> MNQSDSSLMDLPLEIHLSLLEYVPNELRAVNKYFYVLHNHSYKEKSLAWI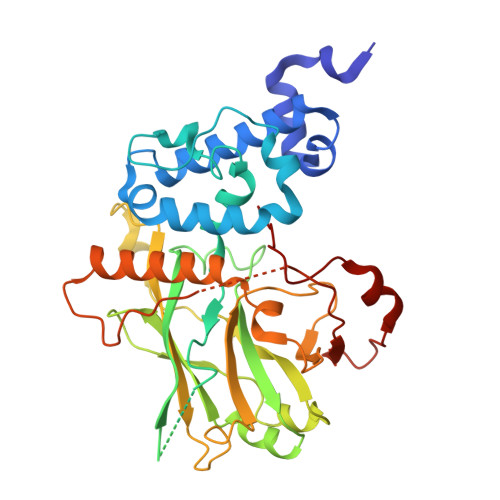AEDNYIWAVVKHSLCLYVKSLDPLRQHAREIIQETKEPGFNVPLCMTKYIADSWYIVYNALQYPGKIINMGWDKYTKSQDLNGSDSTSNFNSRPKERTLMQSLTALPVNFWSRKKDEPTPVNVWFYVKNAHVARYIPKIITEIGICNYGPKQIVASAGYINELITSEGIYCVNLGHLPRLYDEQIFEGTGTTHLPLELKAIDRTDSDVCINSDLVLLGYDFIPYQISKPWLLFRIEPVNSIEAIFNYSECSFSYQFAWSLACLQSEEKISFPRDTIIGHGLPYKPSKLIRIFVYKHPEQKQDLGQEIALPNWNTPYLRR>SLTTTEVVMENVTAFWEEGGTPVLKDINFKIERGQLLAVAGSTGAGKTSLLMMIMGELEPSEGKIKHSGRISFCSQFSWIMPGTIKENIIFGVSYDEYRYRSVIKACQLEEDISKFAEKDNIVLGEGGITLSGG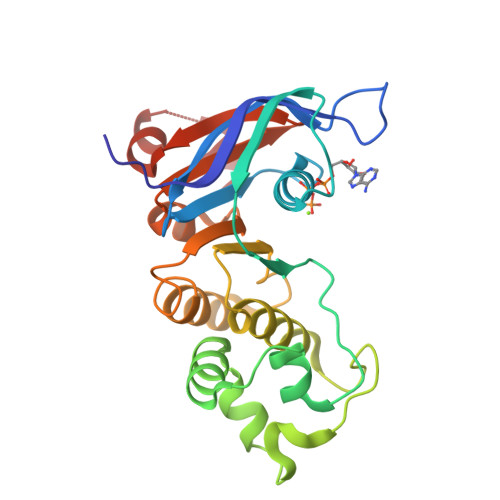QRARISLARAVYKDADLYLLDSPFGYLDVLTEKEIFESCVCKLMANKTRILVTSKMEHLKKADKILILHEGSSYFYGTFSELQNLQPDFSSKLMG[2x]>[2x]GSMRGKVSL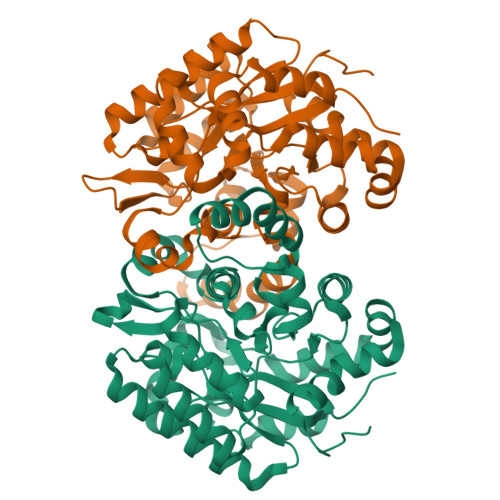EEAFELPKFAAQTKEKAELYIAPNNRDRYFEEILNPCGNRLELSNKHGIGYTIYSIYSPGPQGWTERAECEEYARECNDYISGEIANHKDRMGAFAALSMHDPKQASEELTRCVKELGFLGALVNDVQHAGPEGETHIFYDQPEWDIFWQTCVDLDVPFYLHPEPPFGSYLRNQYEGRKYLIGPPVSFANGVSLHVLGMIVNGVFDRFPKLKVILGHLGEHIPGDFWRIEHWFEHCSRPLAKSRGDVFAEKPLLHYFRNNIWLTTSGNFSTETLKFCVEHVGAERILFSVDSPYEHIDVGCGWYDDNAKAIMEAVGGEKAYKDIGRDNAKKLFKLGKFYDSEA> MSAPTPLAEASQIPTIPALSPLTAKQSKGNFFSSNPISSFVVDTYKQLHSHRQSLELVNPGTVENLNKEVSRDVFLSQYFFTGLRADLNKAFS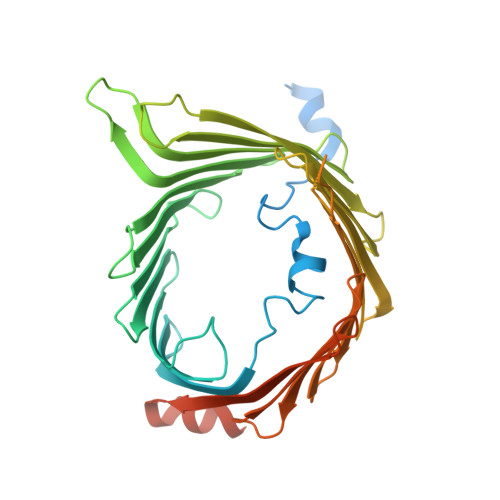MNPAFQTSHTFSIGSQALPKYAFSALFANDNLFAQGNIDNDLSVSGRLNYGWDKKNISKVNLQISDGQPTMCQLEQDYQASDFSVNVKTLNPSFSEKGEFTGVAVASFLQSVTPQLALGLETLYSRTDGSAPGDAGVSYLTRYVSKKQDWIFSGQLQANGALIASLWRKVAQNVEAGIETTLQAGMVPITDPLMGTPIGIQPTVEGSTTIGAKYEYRQSVYRGTLDSNGKVACFLERKVLPTLSVLFCGEIDHFKNDTKIGCGLQFETAGNQELLMLQQGLDADGNPLQALPQLGGWSHPQFEK>MSENAEPVSKLRIRTPSGEFLERRFLASNKLQIVFDFVASKGFPWDEYKLLSTFPRRDVTQLDPNKSLLEVKLFPQETLFLEA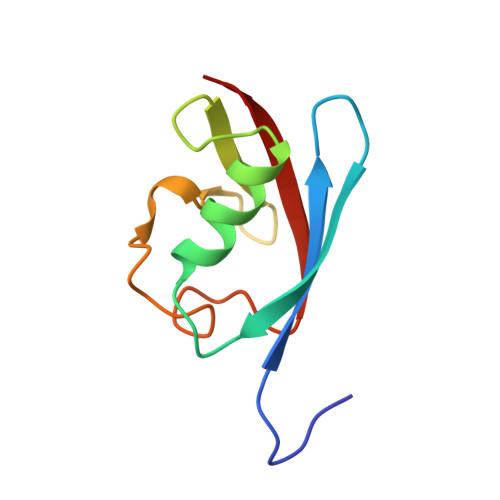KE[4x]The L-arginine biosynthesis pathway consists of eight enzymes that catalyse the conversion of L-glutamate to L-arginine, appears to be attractive target for anti-Tuberculosis (TB) drug discovery. The arginine biosynthesis pathway consists of eight different enzymes ([Fig fig1]) all considered to be essential for *M. tuberculosis* growth *in vitro*. In this work, the ligandability of four enzymes of the pathway ArgB, ArgC, ArgD and ArgF is explored using a fragment-based approach. In conclusion, using a fragment-based approach, we have discovered inhibitors that bind to novel sites in ArgB and ArgF and to the active sites of ArgC and ArgD, which in case of ArgB show on target activity against *M. tuberculosis*.

(A) X-ray crystal structure of ArgC apoenzyme superposed with the NAPD bound holoenzyme. Binding of NAPD causes significant structural changes in two loops of the protein that move from a closed to open conformation ([Fig fig2]). The apoenzyme ArgC with 5% DMSO was found to have a melting temperature of 67.7 °C. While 1 mM NADP^+^ gave a small average positive thermal shift of ~0.6 °C and 1 mM NADPH produced an average negative thermal shift of −0.9 °C across all DSF runs performed.

>GSMQNRQVANATKVAVAGASGYAGGEILRLLLGHPAYADGRLRIGALTAATSAGSTLGEHHPHLTPLAHRVVEPTEAAVLGGHDAVFLALPHGHSAVLAQQLSPETLIIDCGADFRLTDAAVWERFYGSSHAGSWPYGLPELPGARDQLRGTRRIAVPGCYPTAALLALFPALAADLIEPAVTVVAVSGTSGAGRAATTDLLGAEVIGSARAYNIAGVHRHTPEIAQGLRAVTDRDVSVSFTPVLIPASRGILATCTARTRSPLSQLRAAYEKAYHAEPFIYLMPEGQLPRTGAVIGSNAAHIAVAVDEDAQTFVAIAAIDNLVKGTAGAAVQSMNLALGWPETDGLSVVGVAP[2x]> GSPREKVAMEYLQSASRVLTRSQLRDVVASSHLLQSEFMEIPMNFVDPKEIDIPRHGTKNRYKTILPNPLSRVCLRPKNITDSLSTYINANYIRGYSGKEKAFIATQGPMINTVNDFWQMVWQEDSPVIVMITKLKEKNEKCVLYWPEKRGIYGKVEVLVTGVTECDNYTIRNLVLKQGSHTQHVKHYWYTSWPDHKTPDSAQPLLQL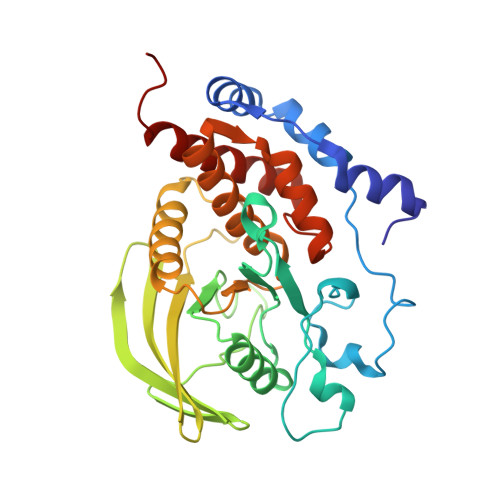MLDVEEDRLASEGRGPVVVHCSAGIGRTGCFIATSIGCQQLKEEGVVDALSIVCQLRVDRGGMVQTSEQYEFVHHALCLFESRLSPETV> MPSPTTVPVATAGRLAEPYIDPAAQVHAIASIIGDVRIAAGVRVAAGVSIRADEGAPFQVGKESILQEGAVIHGLEYGRVLGDDQADYSVWIGQRVAITHKALIHGPAYLGDDCFVGFRSTVFNARVGA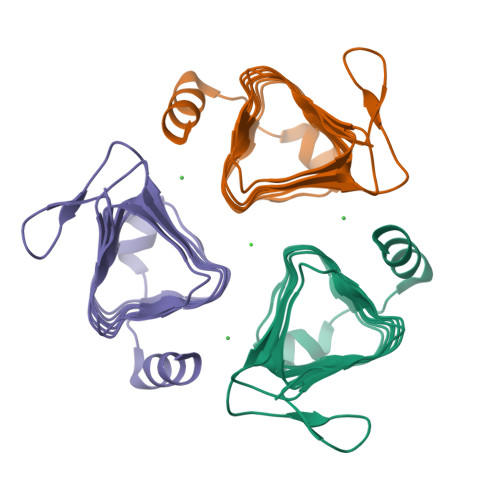GSVIMMHALVQDVEIPPGRYVPSGAIITTQQQADRLPEVRPEDREFARHIIG> MATLGHTFPFYAGPKPTFPMDTTLASIIMIFLTALATFIVILPGIRGKTRLFWLLRVVTSLFIGAAILAVNFSSEWSVGQVSTNTSYKAFSSEWISADIGLQVGLGGVNITLTGTPVQQLNETINYNEEFTWRLGENYAEEYAKALEKGLPDPVLYLAEKFTPRSPCGLYRQYRLAGHYTSAMLWVAFLCWLLANVMLSMPVLVYGGYMLLATGIFQLLALLFFSMATSLTSPCPLHLGASVLHTHHGPAFWITLTTGLLCVLLGLAMAVAHRMQPHRLKAFFNQSVDEDPMLEWSPEEGGLLSPRYRSMADSPKSQDIPLSEASSTKAYYRPRRLSLVPADVRGLAPAALSALPGALLAQAWRALLPGLRCPKAGKESRLGPPHSPWRFGPEGCEERWAEHTGDSPRPLRGRGTGRLWRWGSKERRACGVRAMLPRLVSNSGLKRPSCLDLPKCWDYRRDARAFFHLLEPTPCVTSRHT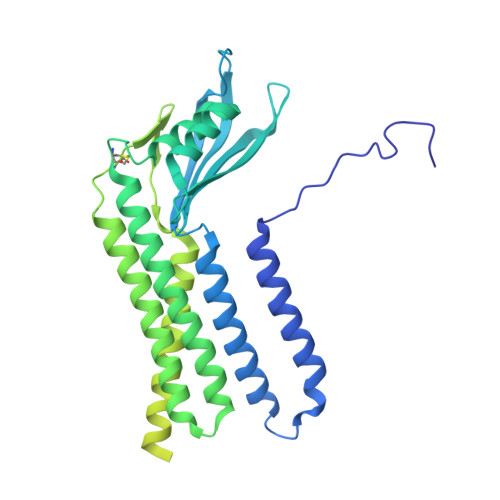PLI{(2S,5R,6S)-6-(3-chlorophenyl)-5-(4-chlorophenyl)-4-[(2S)-1-hydroxybutan-2-yl]-3-oxomorpholin-2-yl}acetic 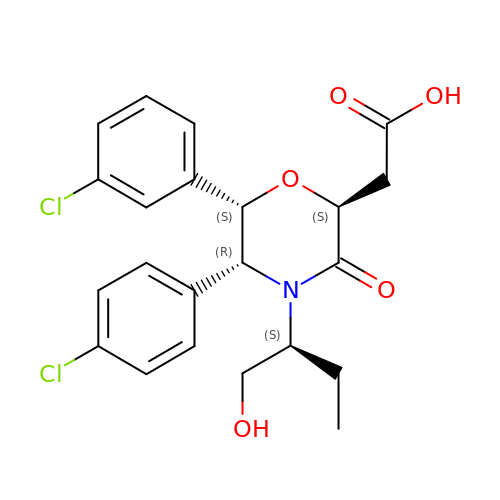acid | C22 H23 Cl2 N O5 | GOJFTLJDUNFYCJ-MMKMLUHNSA-N6-methyl-4-oxidanyl-pyran-2-one | C6 H6 O3 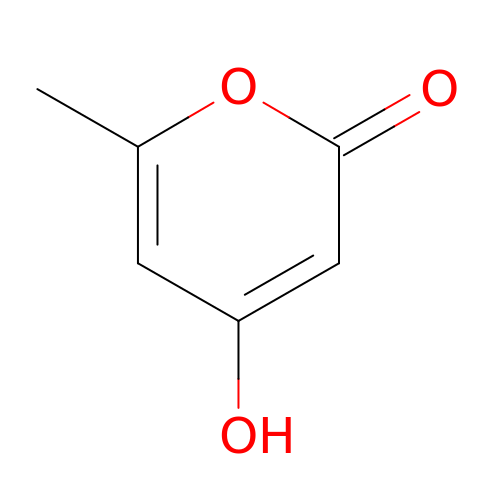| NSYSSMYQPLSPOD-UHFFFAOYSA-N>MPCRLTRLFGIEFPIIQAPMAGVQGSALAIAVSEAGGLGSLPCAMLSLEALEAELTAIRSQTAKPINVNFFCHREPVAQAAKQAAWLEQLAPYFAEFNLDPNAQPAGAQRTPYSKAQAEVLAKFKPEVVSFHFGLPDEELLLEIKSWGSKVISTATTVEEALWLEARGADAIIAQGLEAGGHRGHFLSEDLTEQLGTFSLLPQIIAAVEIPVIAAGGIVDATTVRAAMTMGASAVQVGTAYLLCPECNTSAIHREALQSDAAQHTALTNLFSGRPARGIVNRFMAEMGPMNEAVPDFPLASSAVAGLRTAAERLGFWDFSPLWCGQNASGCRAIP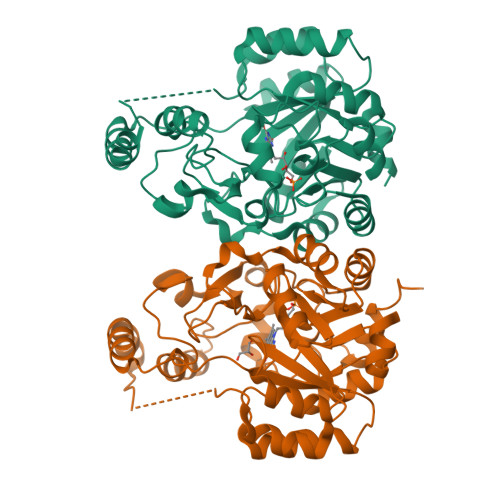AADLTRSFVLSLPSSCVEPQEKSG[8x]>SLMSVDPNYTEMEGKVREATNNEPWGASSTLMDQISQGTYNFREREEILSMIFRRFTEKAGSEWRQIYKALQLLDYLIKHGSERFIDDTRNSINLIRILETFHYIDSQGRDQGINVRTRVKALIELLSDDNKIRAERKKARETAKKYKGV[2x];> SLLISYESDFKTTLEQAKASLAEAPSQPLSQRNTTLKHVEQQQDELFDLLDQMDVEVNNSIGDASE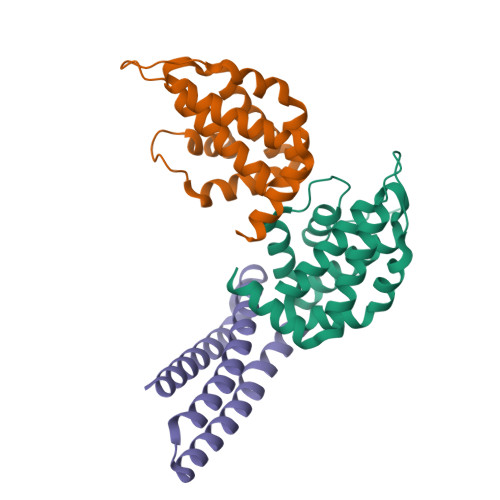RATYKAKLREWKKTIQSDIKRPLQSLVDSGD>[2x]ARVAVLISGTGSNLQALIDSTREPNSSAQIDIVISNKAAVAGLDKA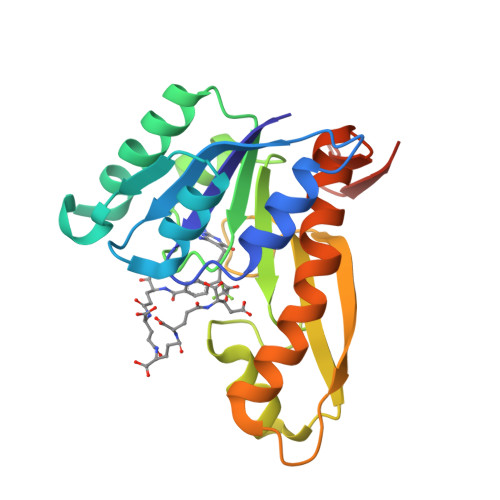ERAGIPTRVINHKLYKNRVEFDSAIDLVLEEFSIDIVCLAGFMRILSGPFVQKWNGKMLNIHPSLLPSFKGSNAHEQALETGVTVTGCTVHFVAEDVDAGQIILQEAVPVKRGDTVATLSERVKLAEHKIFPAALQLVASGTVQLGENGKICWVKEEHHHHHH> MGSSHHHHHHSSGHMEQNPQSQLKLLVTRGKEQGYLTYAEVNDHLPEDIVDSDQIEDIIQMINDMGIQVMEEAPDADDLMLAENTADEDAAEAAAQVLSSVESEIGRTTDPVRMYMREMGTVELLTREGEIDIAKRIEDGINQVQCSVAEYPEAITYLLEQYDRVEAEEARLSDLITGFVDPNAEEDLAPTATHVGSELSQEDLDDDEDEDEEDGDDDSADDDNSIDPELAREKFAELRAQYVVTRDTIKAKGRSHATAQEEILKLSEVFKQFRLVPKQFDYLVNSMRVMMDRVRTQERLIMKLCVEQCKMPKKNFITLFTGNETSDTWFNAAIAMNKPWSEKLHDVSEE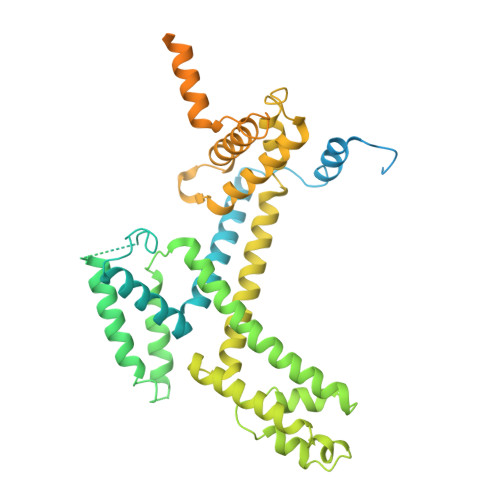VHRALQKLQQIEEETGLTIEQVKDINRRMSIGEAKARRAKKEMVEANLRLVISIAKKYTNRGLQFLDLIQEGNIGLMKAVDKFEYRRGYKFSTYATWWIRQAITRSIADQARTIRIPVHMIETINKLNRISRQMLQEMGREPTPEELAERMLMPEDKIRKVLKIAKEPISMETPIGDDEDSHLGDFIEDTTLELPLDSATTESLCAATHDVLAGLTAREAKVLRMRFGIDMNTDYTLEEVGKQFDVTRERIRQIEAKALRKLRHPSRSEVPRSFLDD>[2x]MGAVIGNESITINSPSTNVESDTKVNVTLAY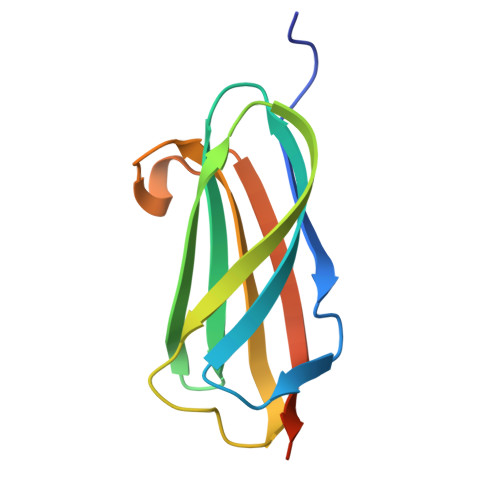TANATRDIVAEFWSSTGWLGQAVKTVSAGNRTETLTINLNNAPATGSGYVVKASIRPVGTNWTSNIATDQVNGLNVIPALEHHHHHH>[2x]MKQNDTKKTTQRRNSKKYSSKTNRGTKRAPRDQEVGTGAQESTRNDVAWYARYPHILEEATRLPFAYPIGQYYDTGYSVASATEWSKYVDTSLTIPGVMCVNFTPTPGESYNKNSPINIAAQNVYTYVRHMNSGHANYEQADLMMYLLAMDSLYIFHSYVRKILAISKLYTPVNKYFPRALLVALGVDPEDVFANQAQWEYFVNMVAYRAGAFAAPASMTYYERHAWMSNGLYVDQDVTRAQIYMFKPTMLWKYENLGTTGTKLVPLMMP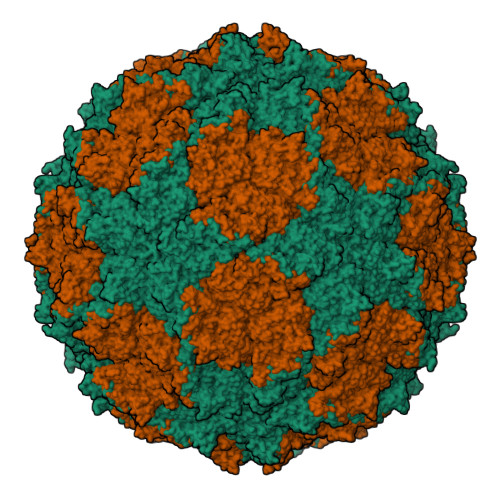KAGDNRKLVDFQVLFNNLVSTMLGDEDFGIMSGDVFKAFGADGLVKLLAVDSTTMTLPTYDPLILAQIHSARAVGAPILETSTLTGFPGRQWQITQNPDVNNGAIIFHPSFGYDGQDHEELSFRAMCSNMILNLPGEAHSAEMIIEATRLATMFQVKAVPAGDTSKPVLYLPNGFGTEVVNDYTMISVDKATPHDLTIHTFFNNILVPNAKENYVANLELLNNIIQFDWAPQLYLTYGIAQESFGPFAQLNDWTILTGETLARMHEVCVTSMFDVPQMGFNK>GPLGSASLQRRSDFCGQWDTATAGDFTLYNDLWGESAGTGSQCTGVDSYSGDTIAWHTSWSWSGGSSSVKSYVNAALTFTPTQLNCISSIPTTWKWSYSGSSIVADVAYDTFLAETASGSSKYEIMVWLAALGGA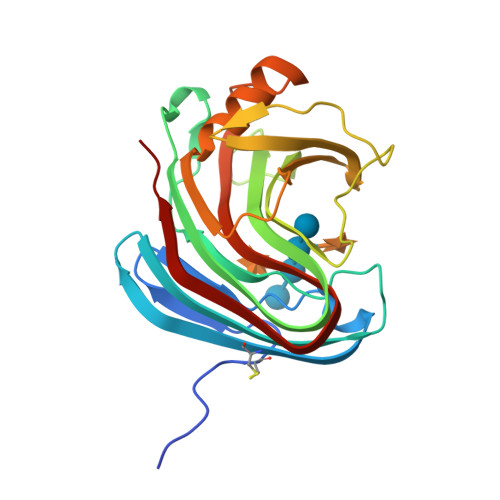GPISSTGSTIATPTIAGVNWKLYSGPNGDTTVYSFVADSTTESFSGDLNDFFTYLVDNEGVSDELYLTTLEAGTEPFTGSNAKLTVSEYSISIE[2x]>[2x]HGGEAHMVPMDKTLKEFGADVQWDDYAQLFTLIKDGAYVKVKPGAQTAIVNGQPLALQVPVVMKDNKAWVSDTFINDVFQSGLDQTFQVEKRPHPLNALTADEIKQAVEIVKASADFKPNTRFTEISLLPPDKEAVWAFALENKPVDQPRKADVIMLDGKHIIEAVVDLQNNKLLSWQPIKDAHGMVLLDDFASVQNIINNSEEFAAAVKKRGITDAKKVITTPLTVGYFDGKDGLKQDARLLKVISYLDVGDGNYWAHPIENLVAVVDLEQKKIVKIEEGPVVPVPMTARPFDGRDRVAPAVKPMQIIEPEGKNYTITGDMIHWRNWDFHLSMNSRVGPMISTVTYNDNGTKRKVMYEGSLGGMIVPYGDPDIGWYFKAYLDSGDYGMGTLTSPIARGKDAPSNAVLLNETIADYTGVPMEIPRAIAVFERYAGPEYKHQEMGQPNVSTERRELVVRWISTVGNYDYIFDWIFHENGTIGIDAGATGIEAVKGVKAKTMHDETAKDDTRYGTLIDHNIVGTTHQHIYNFRLDLDVDGENNSLVAMDPVVKPNTAGGPRTSTMQVNQYNIGNEQDAAQKFDPGTIRLLSNPNKENRMGNPVSYQIIPYAGGTHPVAKGAQFAPDEWIYHRLSFMDKQLWVTRYHPGERFPEGKYPNRSTHDTGLGQYSKDNESLDNTDAVVWMTTGTTHVARAEEWPIMPTEWVHTLLKPWNFFDETPTLGALKKDK

Copper amine oxidases (CuAOs) catalyse the oxidation of a wide range of amine substrates to generate a product aldehyde, ammonia and hydrogen peroxide. In bacteria, they play a role in general nitrogen catabolism. They contain a protein-derived cofactor that is generated autocatalytically by post-translation modification of a conserved endogenous tyrosine to generate 2,4,5-trihydroxylphenylalanine quinone (TPQ), requiring only the presence of copper and molecular oxygen. TPQ is situated in the core of the protein at the end of a well defined substrate-access channel next to a type II copper coordinated by three histidines. ECAO is distinct from Gram positive bacterial and yeast CuAOs in that it possesses an extra 9.3 kDa N-terminal domain, which gives ECAO a characteristic ‘mushroom stalk and cap’ shape.

Bio­chemical and structural characterization of ECAO indicate that the binding of oxygen in the active site is similar to that of the other family members; however, it is possible that the presence of the additional N-terminal domain, which is located at one end of the structurally conserved β-sandwich, could alter or provide an alternate pathway for oxygen entry. In order to investigate this possibility, we have determined the crystal structure of ECAO in complex with xenon at 2.5 Å resolution. The Xe atoms were bound in hydrophobic pockets located in either the amine substrate-entry channel or around the conserved β-sandwich oxygen-entry pathway. Nearly identical sites were observed in both subunits of ECAO present in the asymmetric unit1. Two Xe atoms are bound in the amine substrate-entry channel. Xenon 4/11 occupies a site between Tyr381 and Tyr387 that is equivalent to that previously observed in AGAO and HPAO. We did not observe any xenon-binding sites inside the lower half of the β-sandwich near the ‘bottom’ entrance to the putative oxygen-entry pathway. A final xenon, xenon –/10, is bound at the edge of ECAO in a hydrophobic pocket and is not close to any previously observed xenon position. No xenon-binding sites are observed in the ECAO N-­terminal domain itself nor does the presence of this domain appear to affect xenon binding in the lower half of the β-sandwich when compared with other CuAOs for which xenon complexes have been determined. These observations indicate that the N-terminal domain does not play a role in oxygen entry during ECAO catalysis, which is consistent with the lack of conservation of the N-terminal domain across the CuAOs.>GLNFPTYDGKDRVVSLTEKNFKQVLKKYDVLCLYYHESVSSDKVAQKQFQLKEIVLELVAQVLEHKDIGFVMVDAKKEAKLAKKLGFDEEGSLYVLKGDRTIEFDGEFAADVLVEFLLDLIEDPVEIINSKLEVQAFERIEDQIKLIGFFKSEESEYYKAFEEAAEHFQPYIKFFATFDKGVAKKLSLKMNEVDFYEPFMDEPIAIPDKPYTEEELVEFVKEHQRPTLRRLRPEDMFETWEDDLNGIHIVAFAERSDPDGYEFLEILKQVARDNTDNPDLSIVWIDPDDFPLLVAYW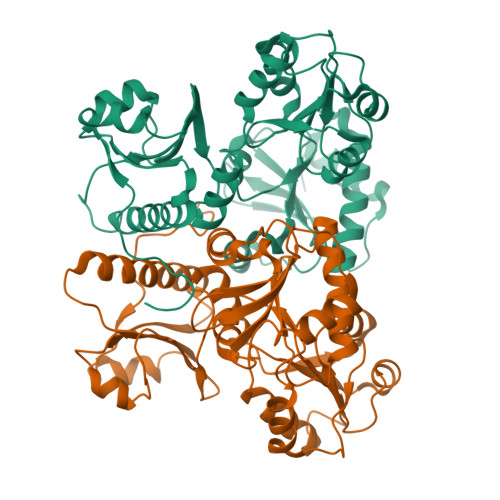EKTFKIDLFKPQIGVVNVTDADSVWMEIPDDDDLPTAEELEDWIEDVLSGKIN[2x]> GEFEKLEALEQLQSHIEGWEGSNLTDICTQLLLQGTLLKISAGNIQERAFFLFDNLLVYCKRKSRVTGSKKSTKRTKSINGSLYIFRGRINTEVMEVENVEDGTADYHSNGYTVTNGWKIHNTAKNKWFVCMAKTAEEKQKWLDAIIREREQRESLKLGME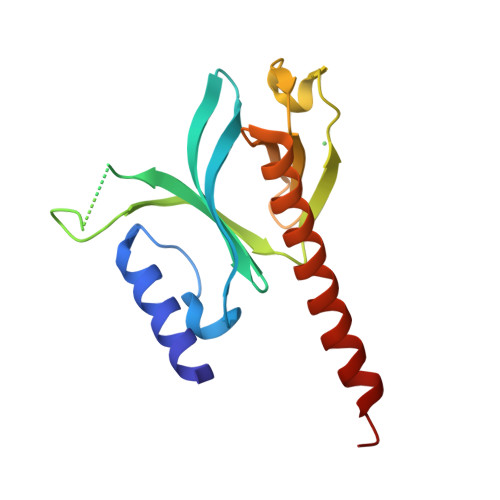RDAYVM>[4x]MGSSHHHHHHSSGLVPRGSSFPDYYEDSLAVIGISCEFPGAKDHYEFWNNIKEGKESITFFSKEELRRSGISEELADHPGFVPAKSVLEGKEMFDPGFFGFSPKDAEYMDPQL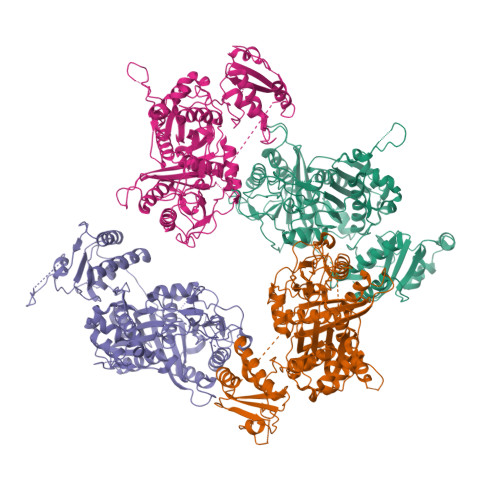RMLLLHSWKAIEDAGYISKEIPETSVYMSASTNSYRSLLPEETTAQLETPDGYVSWVLAQSGTIPTMISHKLGLKGPSYFVHANCSSSLIGLHSAFQSLQSGEAKYALVGGATLHTESSAGYVHQPGLNFSSDGHIKAFDADADGMIGGEGAGAVLLKKASDAVKDGDHIYALLRGIGVNNDGADKVGFYAPSVKGQAEVIQKVIDQTGIHPETIAYVEAHGTGTKLGDPIELSALQSVYGRYTDKKQYCGIGSVKTNLGHLDTAAGMAGCIKVVMSLYHQEIAPSINYKEPNPNLHLEDSPFFVAEEKKELTRENRAHRMALSSFGLGGTNTHAIFEQYPDASEAADAAGPFIIPLSARKKDRLKEYAKQLLAFLERKTDTDLADLAYTFQVGREAMEERAAFITSGTAELKRQLADFINDKPAVTGCFRGEKQQAKDIAWLSDDDDSAELIEKWLAKGKGPKLCEMWSKGVAINWHKLYKDKHPKRISLPVYPFAKEPYWPKKAEKN>[2x]MAGIAMKLAKDREAAEGLGSHERAIKYLNQDYETLRNECLEAGALFQDPAFPPVSHSLGFKELGPNSSKTYGIKWKRPTELLSNPQFIVDGATRTDICQGALGDSWLLAAIASLTLNETILHRVVPYGQSFQEGYAGIFHFQLWQFGEWVDVVVDDLLPTKDGKLVFVHSAQGNEFWSALLEKAYAKVNGSYEALSGGCTSEAFEDFTGGVTEWYDLQKAPSDLYQIILKALERGSLLGCSINISDIRDLEAITFKNLVRGHAYSVTDAKQVTYQGQRVNLIRMRNPWGEVEWKGPWSDNSYEWNKVDPYEREQLRVKMEDGEFWMSFRDF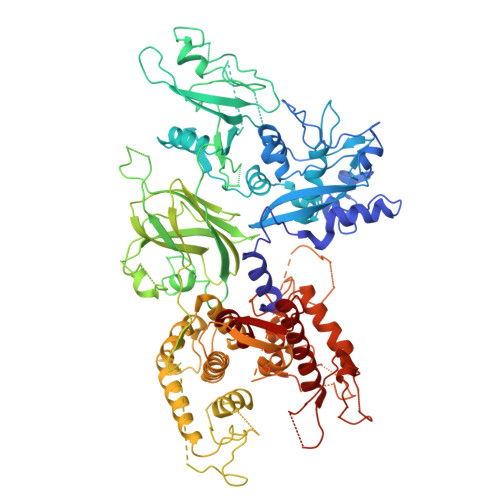IREFTKLEICNLTPDALKSRTLRNWNTTFYEGTWRRGSTAGGCRNYPATFWVNPQFKIRLEEVDDADDYDSRESGCSFLLALMQKHRRRERRFGRDMETIGFAVYQVPRELAGQPVHLKRDFFLANASRAQSEHFINLREVSNRIRLPPGEYIVVPSTFEPNKEGDFLLRFFSEKKAGTQELDDQIQANLPDEKVLSEEEIDDNFKTLFSKLAGDDMEISVKELQTILNRIISKHKDLRTNGFSLESCRSMVNLMDRDGNGKLGLVEFNILWNRIRNYLTIFRKFDLDKSGSMSAYEMRMAIEAAGFKLPCQLHQVIVARFADDELIIDFDNFVRCLVRLEILFKIFKQLDPENTGTIQLDLISWLSFSVLGKLAAAIEHHHHHHMHYSNIEANESEEERQFRKLFVQLAGDDMEVSATELMNILNKVVTRHPDLKTDGFGIDTCRSMVAVMDSDTTGKLGFEEFKYLWNNIKKWQGIYKRFETDRSGTIGSNELPGAFEAAGFHLNQHIYSMIIRRYSDETGNMDFDNFISCLVRLDAMFRAFRSLDKNGTGQIQVNIQEWLQLTMYS> PTQCDVPPNSRFDCAPDKAITQEQCEARGCCYIPAKQGLQGAQMGQPWCFFPPSYPSYKLENLSSSEMGYTATLTRTTPTFFPKDILTLRLDVMMETENRLHFTIKDPANRRYEVPLETPHVHSRAPSPLYSVEFSEEPFGVIVHRQLDGRVLLNTTVAPLFFADQFLQLSTSLPSQYITGLAEHLSPLMLSTSWTRITLWNRDLAPTPGANLYGSHPFYLALEDGGSAHGVFLLNSNAMDVVLQPSPALSWRSTGGILDVYIFLGPEPKSVVQQYLD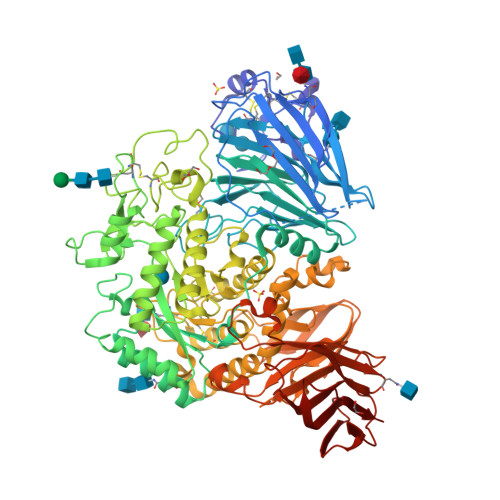VVGYPFMPPYWGLGFHLCRWGYSSTAITRQVVENMTRAHFPLDVQWNDLDYMDSRRDFTFNKDGFRDFPAMVQELHQGGRRYMMIVDPAISSSGPAGSYRPYDEGLRRGVFITNETGQPLIGKVWPGSTAFPDFTNPTALAWWEDMVAEFHDQVPFDGMWIDMNEPSNFIRGSEDGCPNNELENPPYVPGVVGGTLQAATICASSHQFLSTHYNLHNLYGLTEAIASHRALVKARGTRPFVISRSTFAGHGRYAGHWTGDVWSSWEQLASSVPEILQFNLLGVPLVGADVCGFLGNTSEELCVRWTQLGAFYPFMRNHNSLLSLPQEPYSFSEPAQQAMRKALTLRYALLPHLYTLFHQAHVAGETVARPLFLEFPKDSSTWTVDHQLLWGEALLITPVLQAGKAEVTGYFPLGTWYDLQTVPIEALGSLPPPPAAPREPAIHSEGQWVTLPAPLDTINVHLRAGYIIPLQGPGLTTTESRQQPMALAVALTKGGEARGELFWDDGESLEVLERGAYTQVIFLARNNTIVNELVRVTSEGAGLQLQKVTVLGVATAPQQVLSNGVPVSNFTYSPDTKVLDICVSLLMGEQFLVSWC METHYL 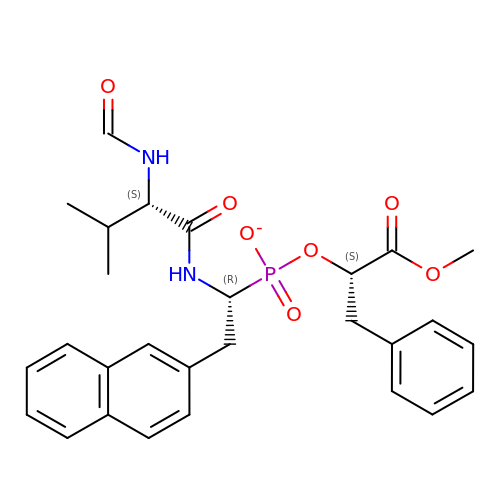(2S)-[1-((N-FORMYL)-L-VALYL)AMINO-2-(2-NAPHTHYL)ETHYL)HYDROXYPHOSPHINYLOXY]-3-PHENYL PROPANOATE | C28 H32 N2 O7 P | SBIPQEWAZQAMRY-NXCFDTQHSA-M(PHENYL-PHOSPHONO-METHYL)-PHOSPHONIC ACID | C7 H10 O6 P2 | 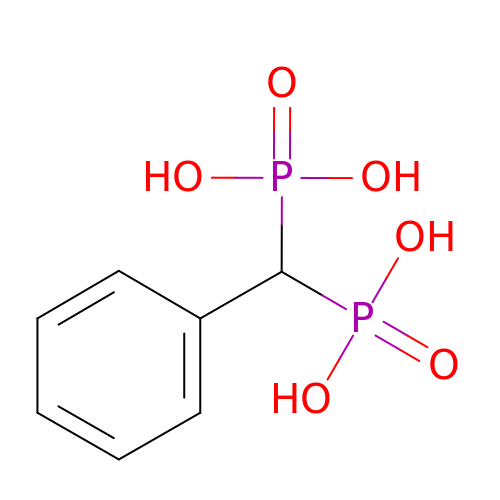FRLTXWJJMCIUNT-UHFFFAOYSA-N>[10x]TPQNITDLCAEYHNTQIHTLNDKIFSYTESLAGKREMAIITFKNGATF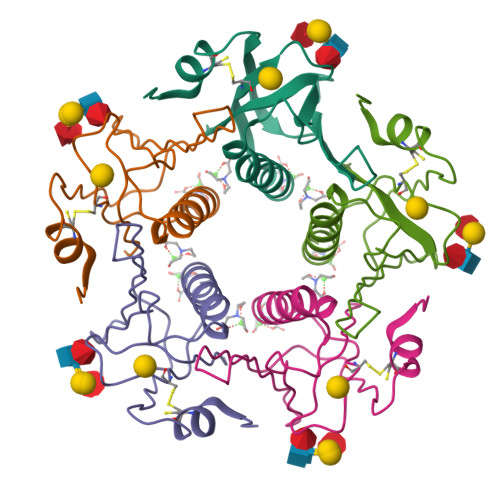QVEVPGSQHIDSQKKAIERMKDTLRIAYLTEAKVEKLCVWNNKTPHAIAAISMAN5-CHLORO-THIOPHENE-2-CARBOXYLIC ACID 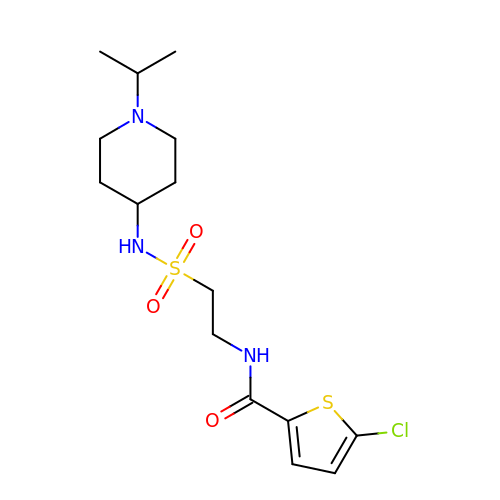[2-(1--ISOPROPYL-PIPERIDIN-4-YLSULFAMOYL)-ETHYL]-AMIDE | C15 H24 Cl N3 O3 S2 | XIOBNAKYNXSFFO-UHFFFAOYSA-N>[2x]MSGNMDEAVSGNMDEAVSAGKDVRIARWVATIAGLLGFVLSVSIPLLPVTQTTATLNWPQQGRLDNVTAPLISQAPLELTATVPCSVVRDLPPEGGLVFGTAPAEGRDAALNAMLVNVTETRVDVIVRNVVVASVNRDRVAGPDCQRIEITSNLDGTYADFVGLTQISGEDAGKLQRTGYPDPNLRPAIVGVFTDLTGPAPQGLSVSAEIDTRFTTHPTALKLAAMLLAIVSTVIALLALWRLDRLDGRRMHRLIPTRWRTVTAVDGVVVGGMAIWYVIGANSSDDGYILQMARTAEHAGYMANYFRWFGSPEDPFGWYYNVLALMTKVSDASIWIRLPDLICALICWLLLSREVLPRLGPAVAGSRAAMWAAGLVLLGAWMPFNNGLRPEGQIATGALITYVLIERAVTSGRLTPAALAITTAAFTLGIQPTGLIAVAALLAGGRPILRIVMRRRRLVGTWPLIAPLLAAGTVILAVVFADQTIATVLEATRIRTAIGPSQEWWTENLRYYYLILPTTDGAISRRVAFVFTAMCLFPSLFMMLRRKHIAGVARGPAWRLMGIIFATMFFLMFTPTKWIHHFGLFAAVGGAMAALATVLVSPTVLRSARNRMAFLSLVLFVLAFCFASTNGWWYVSNFGAPFNNSVPKVGGVQISAIFFALSAIAALWAFWLHLTRRTESRVVDRLTAAPIPVAAGFMVVVMMASMAIGVVRQYPTYSNGWANIRAFAGGCGLADDVLVEPDSNAGFLTPLPGAYGPLGPLGGEDPQGFSPDGVPDRIIAEA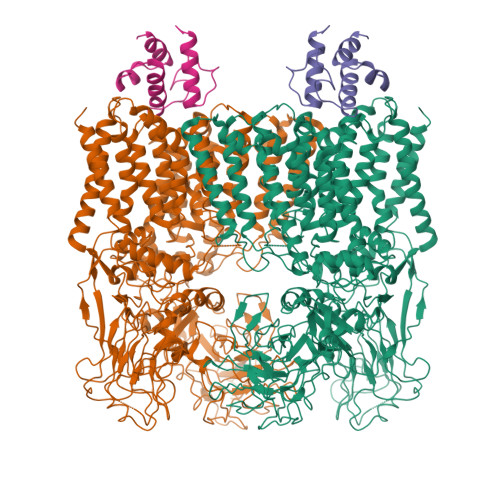IRLNNPQPGTDYDWNRPIKLDEPGINGSTVPLPYGLDPKRVPVAGTYSTEAQQESRLSSAWYELPARDETERAAHPLVVITAAGTITGESVANGLTTGQTVDLEYATRGPDGTLVPAGRVTPYDVGPTPSWRNLRYPRSEIPDDAVAVRVVAEDLSLSQGDWIAVTPPRVPELQSVQEYVGSDQPVLMDWAVGLAFPCQQPMLHANGVTEVPKFRISPDYYAKLQSTDTWQDGINGGLLGITDLLLRASVMSTYLSQDWGQDWGSLRKFDTVVEATPAELDFGSQTHSGLYSPGPLRIRP;>[2x]MAATQEEIIAGLAEIIEEVTGIEPSEVTPEKSFVDDLDIDSLSMVEIAVQTEDKYGVKIPDEDLAGLRTVGDVVAYIQKLEEENPEAAAALREKFAADQ>MIIERLVGNLRDLNPLDFSVDHVDLEWFETRKKIARFKTRQGKDIAIRLKDAPKLGLSQGDILFKEEKEIIAVNILDSEVIHIQAKSVAEVAKICYEIGNRHAALYYGESQFEFKTPFEKPTLALLEKLGVQNRVLSSKLDSKERLTVSMPHSEPN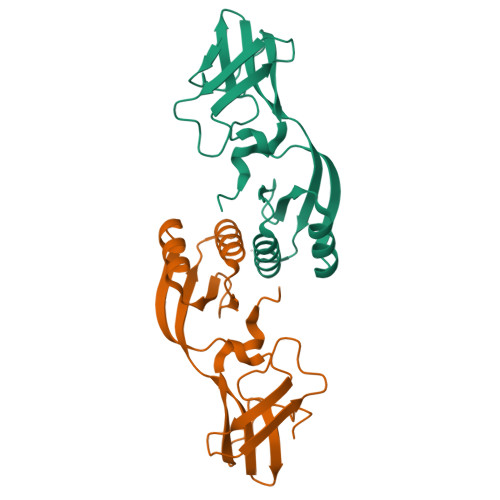FKVSLASDFKVVVK[4x]> MDKRRVVVTGIGAVTPIGNDAETSWENAKKGVNGVAKMTRLNPDDFPVKIAAELKDFDVEKYLEKKEARKMDRFTHYAIASAEMAVQDSGLVIDDSNANRVGVWI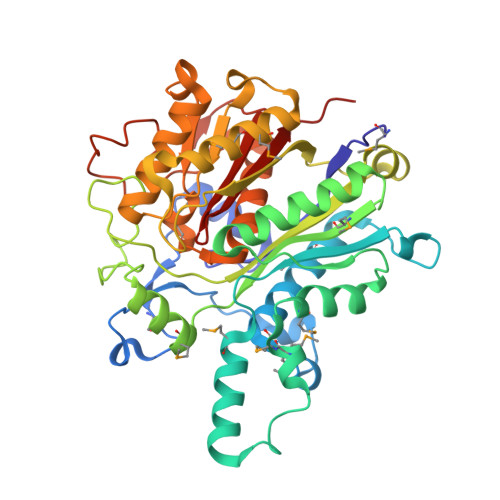GSGIGGMETFETQYEIFLNRGHRRVSPFFVPMMIPDMGSGQVSIRFGAKGINSTTVTACATATNSIGDAFKVIERGDADAMITGGAEAPITKMSLAGFTANKALSLNPDPETACRPFDKDRDGFIIGEGAGIVILEEYEHAKARGAKIYAEIVGYGATGDAYHITAPAPNGEGAARAMKMAIDDAGLTPDKVDYINAHGTSTPYNDEYETQAIKTVFGEHAKKLAISSTKSMTGHTLGASGGIEAIFALLTIRDNIIAPTIHLKNQDEVCDLDYVPNEAREANVNVVISNSFGFGGHNATLVFKRIED> ASFGSRLEDAVKKTVAENPVVVYSKTWCSYSSEVKSLFKRLNVDPLVVELDELGAQGPQIQKVLERLTGQHTVPNVFIGGKHIGGCTDTVKLYRKGELEP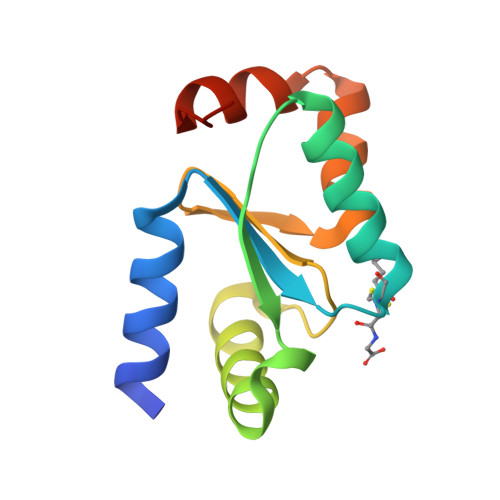LLSEANAKKSQG> MGSSHHHHHHSSGLVPRGSMSTSWSDRLQNAADMPANMDKHALEKYRREAYHRVFVNRSLAMEKIKCFGFDMDYTLAVYKSPEYESLGFELTVERLVSIGYPQELLSFAYDSTFPTRGLVFDTLYGNLLKVDAYGNLLVCAHGFNFIRGPETREQYPNKFIQRDDTERFYILNTLFNLPETYLLACLVDFFTNCPRYTSCETGFKDGDLFMSYRSMFQDVRDAVDWVHYKGSLKEKTVENLEKYVVKDGKLPLLLSRMKEVGKVFLATNSDYKYTDKIMTYLFDFPHGPKPGSSHRPWQSYFDLILVDARKPLFFGEGTVLRQVDTKTGKLKIGTYTGPLQHGIVYSGGSSDTICDLLGAKGKDILYIGDHIFGDILKSKKRQGWRTFLVIPELAQELHVWTDKSSLFEELQSLDIFLAELYKHLDSSSNERPDISSIQRRIKKVTHDMDMCYGMMGSLFRS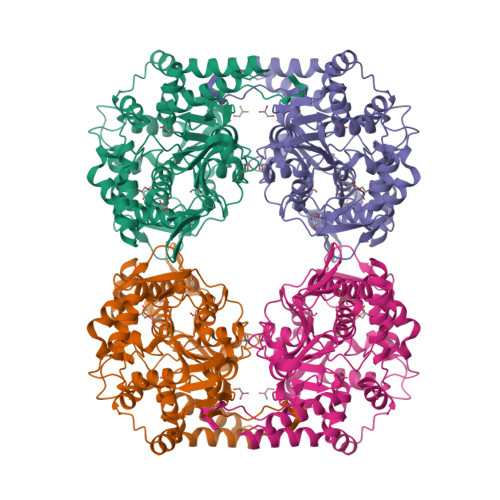GSRQTLFASQVMRYADLYAASFINLLYYPFSYLFRAAHVLMPHESTVEHTHVDINEMESPLATRNRTSVDFKDTDYKRHQLTRSISEIKPPNL> MLLPWLILIPFIGGFLCWQTERFGVKVPRWIALITMGLTLALSLQLWLQGGYSLTQSAGIPQWQSEFDMPWIPRFGISIHLAIDGLSLLMVVLTGLLG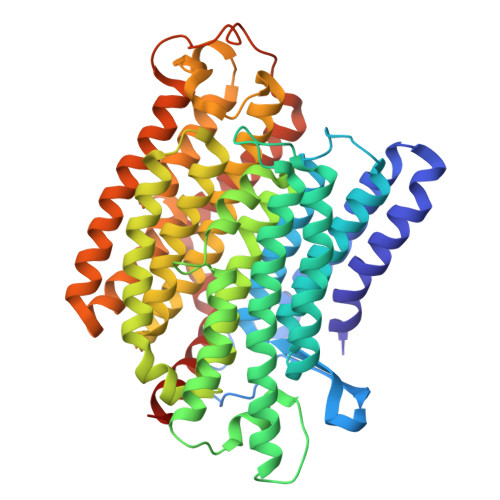VLAVLCSWKEIEKYQGFFHLNLMWILGGVIGVFLAIDMFLFFFFWEMMLVPMYFLIALWGHKASDGKTRITAATKFFIYTQASGLVMLIAILALVFVHYNATGVWTFNYEELLNTPMSSGVEYLLMLGFFIAFAVKMPVVPLHGWLPDAHSQAPTAGSVDLAGILLKTAAYGLLRFSLPLFPNASAEFAPIAMWLGVIGIFYGAWMAFAQTDIKRLIAYTSVSHMGFVLIAIYTGSQLAYQGAVIQMIAHGLSAAGLFILCGQLYERIHTRDMRMMGGLWSKMKWLPALSLFFAVATLGMPGTGNFVGEFMILFGSFQVVPVITVISTFGLVFASVYSLAMLHRAYFGKAKSQIASQELPGMSLRELFMILLLVVLLVLLGFYPQPILDTSHSAIGNIQQWFVNSVTTTRP>MESYHKPDQQKLQALKDTANRLRISSIQATTAA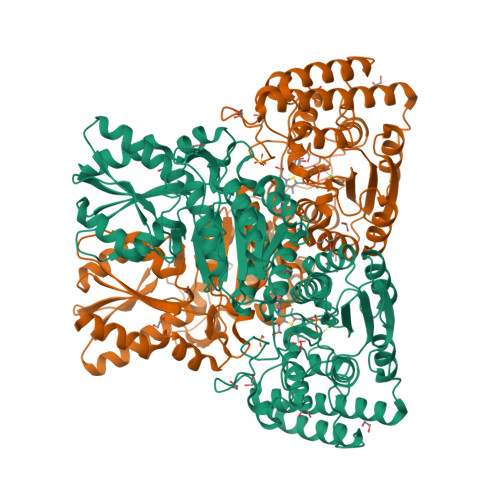GSGHPTSCCSAAEIMAVLFFHTMRYKSQDPRNPHNDRFVLSKGHAAPILYAVWAEAGFLAEAELLNLRKISSDLDGHPVPKQAFTDVATGSLGQGLGAACGMAYTGKYFDKASYRVYCLLGDGELSEGSVWEAMAFASIYKLDNLVAILDINRLGQSDPAPLQHQMDIYQKRCEAFGWHAIIVDGHSVEELCKAFGQAKHQPTAIIAKTFKGRGITGVEDKESWHGKPLPKNMAEQIIQEIYSQIQSKKKILATPPQEDAPSVDIANIRMPSLPSYKVGDKIATRKAYGQALAKLGHASDRIIALDGDTKNSTFSEIFKKEHPDRFIECYIAEQNMVSIAVGCATRNRTVPFCSTFAAFFTRAFDQIRMAAISESNINLCGSHCGVSIGEDGPSQMALEDLAMFRSVPTSTVFYPSDGVATEKAVELAANTKGICFIRTSRPENAIIYNNNEDFQVGQAKVVLKSKDDQVTVIGAGVTLHEALAAAELLKKEKINIRVLDPFTIKPLDRKLILDSARATKGRILTVEDHYYEGGIGEAVSSAVVGEPGITVTHLAVNRVPRSGKPAELLKMFGIDRDAIAQAVRGLITKALVPRGSLEHHHHHH[2x]6-[5-[(1~{R},2~{R},4~{S})-7-azabicyclo[2.2.1]heptan-2-yl]-2-fluoranyl-pyridin-3-yl]pyridine-3-carboxamide | C17 H17 F N4 O | 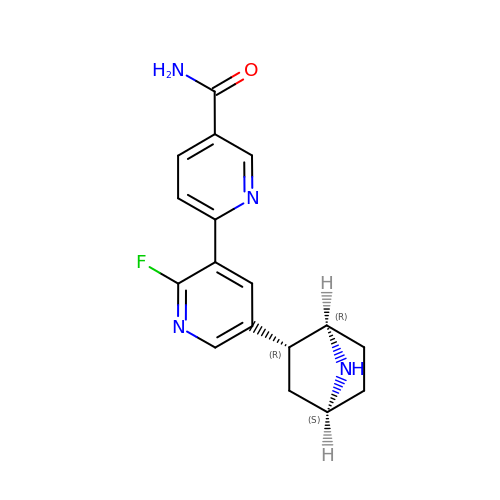OTLVFRDBKUDQLP-YWPYICTPSA-N> MLKRVEIFTDGSCLGNPGPGGYGAILRYRGREKTFSAGYERTTNNRMELMAAIVALEALKEHCEVILSTDSHYVRKGITEWIHNWKKRGWKKADKKPVKNVDLWKRLDAALGQHQIKWEWVKGHAGHPENERCDELARAAAMNPTLEDTG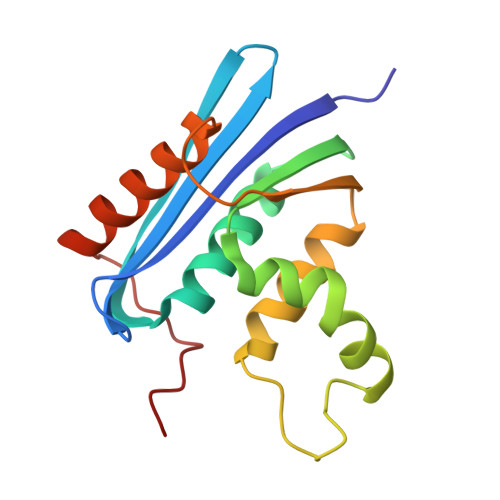YQVEV> MPKTPHTKGPDETLSLLADPYRFISRQCQRLGANAFESRFLLKKTNCLKGAKAAEIFYDTTRFEREGAMPVAIQKTLFGQGGVQGLDGETHRHRKQMFMGLMTPERVRALAQLFEAEWRRAVPGWTRKGEIVFYDELHEPLTRAVCAWAGVPLPDDEAGNRAGELRALFDAAGSASPRHLWSRLARRRVDAWAKRIIEGIRAGSIGSGSGTAAYAIAWHRDRHDDLLSPHVAAVELVNVLRPTVAIAVYITFVAHALQTCSGIRAALVQQPDYAELFVQEVRRFYPFFPAVVARASQDFEWEGMAFPEGRQVVLDLYGSNHDAATWADPQEFRPERFRAWDEDSFNFIPQGGGDHYLGHRCPGEWIVLAIMKVAAHLLVNAMRYDVPDQD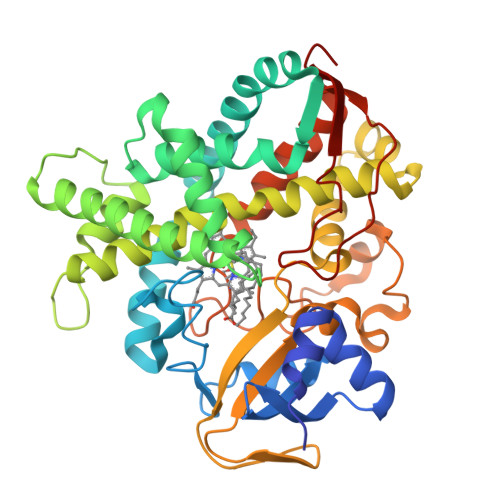LSIDFARLPALPKSGFVMRNVHIGG N-(4-{[6-methoxy-7-(3-morpholin-4-ylpropoxy)quinazolin-4-yl]amino}phenyl)benzamide 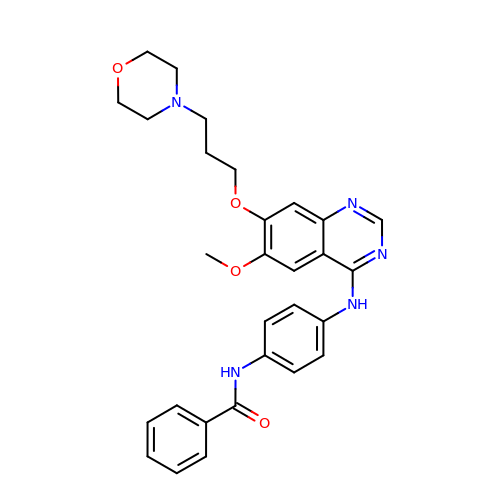| C29 H31 N5 O4 | OGNYUTNQZVRGMN-UHFFFAOYSA-N> MAITADDIAVQYPIPTYRFIVTLGDEQVPFTSASGLDINFDTIEYRDGTGNWFKMPGQRQAPNITLSKGVFPGKNAMYEWINAIQLNQVEKKDI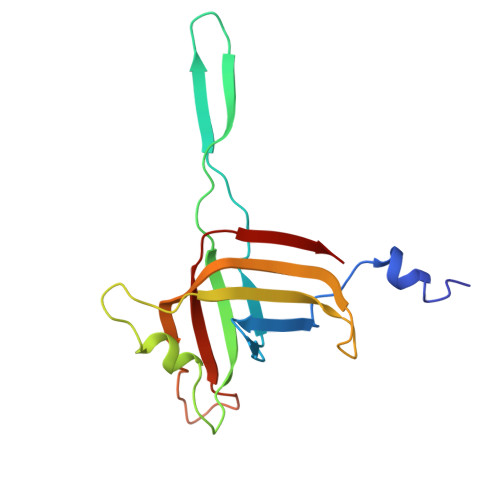MISLTNEAGTEVLVSWNVSNAFPTSLTSPSFDATSNEIAVQQITLMADRVTIQTA> MAGTALKRLMAEYKQLTLNPPEGIVAGPMNEENFFEWEALIMGPEDTXFEFGVFPAILSFPLDYPL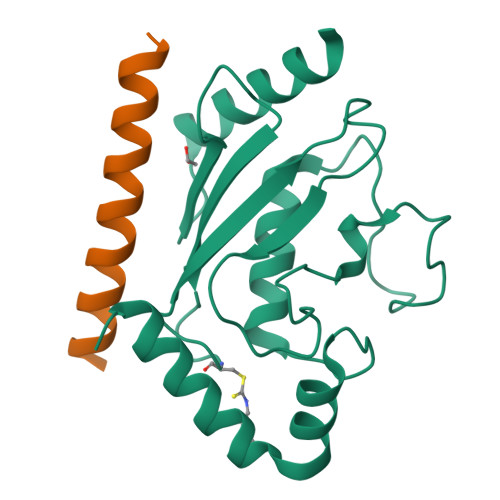SPPKMRFTSEMFHPNIYPDGRVSISILHAPGDDPMGYESSAERWSPVQSVEKILLSVVSMLAEPNDESGANVDASKMWRDDREQFYKIAKQIVQKSLGL;> SADERQRMLVQRKDELLQQARKRFLNK>MEQGICGSHVFFIEDGKSKNYIIGKYKIGYLSGDNLILDPYECLYLYFKGRISFQNSDSFRDLFDTVTFDRYVAYEILKNKGYRVKEDSGLIYFRKGTEKPLSLRVMREYDRIQFSDLVENPVDYYFTVDEEGDPTVYSSQEIFPGGRNLVSPVSAPVVRMGGRSFG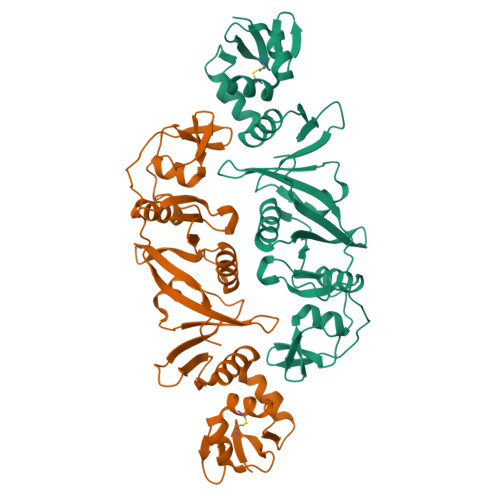AGDLEWWIGTAFHGFRLLTENEANYISGNHSASQVDMVYSDLVGRGCIVKTGFKYGANFRVYLGRDSQHAEYLVSVMPEEERWYSISRGVRVASSVRKTMIYASIYKNEVRYVALKRVKDII[2x]> WTPFSWVEKYAYAFSGPYNKAEVALTFDDGPDLEFTPKILDKLKQHNVKATFFLLGENAEKFPNIVKRIANEGHVIGNHTYSHPNLAKVNEDEYRNQIIKTEEILNRLAGYAPKFIRPPYGEILE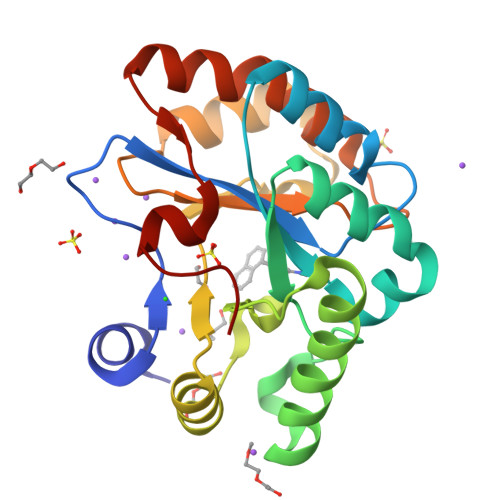NQLKWATEQNFMIVQWSVDTVDWKGVSADTITNNVLGNSFPGSVILQHSTPGGHLQGSVDALDKIIPQLKTKGARFVTLPSMFQTSKER;>[3x]WTPFSWVEKYAYAFSGPYNKAEVALTFDDGPDLEFTPKILDKLKQHNVKATFFLLGENAEKFPNIVKRIANEGHVIGNHTYSHPNLAKVNEDEYRNQIIKTEEILNRLAGYAPKFIRPXYGEILENQLKWATEQNFMIVQWSVDTVDWKGVSADTITNNVLGNSFPGSVILQHSTPGGHLQGSVDALDKIIPQLKTKGARFVTLPSMFQTSKER> GGSMGKTADNHGPVRSETAREGRENQVYSPVTGARLVAGCICLTPDKKQVLMITSSAHKKRWIVPKGGVEKDEPNYETTAQRETWEEAGCIGKIVANLGTVEDMRPPKDWNKDIKQFENSRKDSEVAKHPPRTEFHFYELEIENLLDKFPECHKRHRKLYSYTEAKQNLIDAKRPELLEALNRSAIIKDDK

The yeast diadenosine and diphosphoinositol polyphosphate phosphohydrolase DDP1 is a Nudix enzyme with pyrophosphatase activity on diphosphoinositides, dinucleotides, and polyphosphates. ScDDP1, like its human orthologs, adopts the canonical Nudix fold showing two β sheets flanked by helices. The active site lies in the crevice situated between both β sheets. The longest helix (α-1) contains the Nudix box (GX5EX7REUXEEXGU), which displays a β-loop-helix-loop structure that binds the Mg2+ ions involved in diphosphate moiety orientation and catalysis.

We have defined InsP6 binding as “binding mode 1” (bm1 mode), since its six phosphates make links to the enzyme satisfying all recognition positions, except Pβ of the diphosphate moiety, which is missing in this inositide. In this binding mode, the unique axial phosphate at the 2– position is directed toward the active site. All phosphates participate in one to four interactions with protein residues; thus, P1 makes two (Arg32), P2 makes three (Arg32 bidentate and Gly65 main chain), P3 makes four (Arg152 bidentate and Ser53 side and main chain), P4 makes three (Ser52, Lys63, Arg171), P5 makes three (Arg102 bidentate and Arg129), and P6 makes one (Arg129). Several water-mediated interactions stabilize the inositide. The mentioned residues are involved in the binding of all inositides studied in this work. Focusing on inositide binding, we found seven positions for phosphate recognition: Six positions are defined by the InsP6 complex plus a seventh defined by the “Pβ-to-be-cleaved” position in the PCP-InsP7 complex.>[2x]MVGLEDDTERERSPVVENGFSNGSRSSSSSAGVLSPSRKVTQGNDTLSYANILRARNKFADALALYEAMLEKDSKNVEAHIGKGICLQTQNKGNLAFDCFSEAIRLDPHNACALTHCGILHKEEGRLVEAAESYQKALMADASYKPAAECLAIVLTDLGTSLKLAGNTQEGIQKYYEALKIDPHYAPAYYNLGVVYSEMMQYDNALSCYEKAALERPMYAEAYCNMGVIYKNRGDLEMAITCYERCLAVSPNFEIAKNNMAIALTDLGTKVKLEGDVTQGVAYYKKALYYNWHYADAMYNLGVAYGEMLKFDMAIVFYELAFHFNPHCAEACNNLGVLYKDRDNLDKAVECYQMALSIKPNFAQSLNNLGVVYTVQGKMDAAASMIEKAILANPTYAEAFNNLGVLYRDAGNITMAIDAYEECLKIDPDSRNAGQNRLLAMNYINEGLDDKLFEAHRDWGWRFTRLHPQYTSWDNLKDPERPITIGYISPDFFTHSVSYFIEAPLTHHDYTKYKVVVYSAVVKADAKTYRFRDKVLKKGGVWKDIYGIDEKKIASMVREDKIDILVELTGHTANNKLGTMACRPAPVQVTWIGYPNTTGLPTVDYRITDSLADPPDTKQKQVEELVRLPDCFLCYTPSPEAGPVSPTPALSNGFVTFGSFNNLAKITPKVLQVWARILCAVPNSRLVVKCKPFCCDSIRQRFLTTLEQLGLESKRVDLLPLILFNHDHMQAYSLMDISLDTFPYAGTTTTCESLYMGVPCVTMAGSVHAHNVGVSLLTKVGLGHLVAKNEDEYVQLSVDLASDVTALSKLRMSLRDLMAGSPVCNGPSFAVGLESAYRNMWKKYCKGEVPSLRRMEMLQKEVHDDPLISKDLGPSRVSVTGEATPSLKANGSAPVPSSLPTQSPQLSKRMDSTS

Arabidopsis glycosyltransferase family 41 (GT41) protein SPINDLY (SPY) plays pleiotropic roles in plant development. Despite the amino acid sequence is similar to human O-GlcNAc transferase, Arabidopsis SPY has been identified as a novel nucleocytoplasmic protein O-fucosyltransferase. SPY-like proteins extensively exist in diverse organisms, indicating that O-fucosylation by SPY is a common way to regulate intracellular protein functions. Later studies show that SPY plays important roles in multiple developmental processes, including the circadian clock, phytohormone cytokinin signaling, plant architecture, root development, abiotic and biotic stresses.

Here, we present a crystal structure of Arabidopsis SPY/GDP complex at 2.85 Å resolution. Taken together, sequence alignment, SEC-Mals analysis and enzymatic assays collectively demonstrate that the crystal structure of engineered SPYC645S represents the conformation of wild type SPY. In the crystal structure, two SPY molecules interact with each other in a head-to-tail manner, forming a symmetrical dimer with a length of ~150 Å, a width of ~70 Å and a height of ~75 Å. Eleven tetratricopeptide repeats (TPRs) (residues 44–430) make up a superhelical conformation. The catalytic domain (residues 483–847) comprises the N-terminal lobe (N-Cat) and the C-terminal lobe (C-Cat). A short C-terminal region following the catalytic domain (residues 848–914) is invisible in the structure due to less of density map. GDP is observed on the surface of C-Cat adjacent to the interface with N-Cat. During the model building of our Arabidopsis SPY/GDP complex structure, strikingly, we found that the N-terminal loop of one protomer in a symmetry-related SPY dimer B, encompassing the residues from F20* to S37*, wrapped around the concave surface of the superhelix and traverse the active site of one protomer in the SPY dimer A. More interestingly, S21* in dimer B is located close to the phosphate groups of the GDP in one active site of dimer A, strongly suggesting it is a target residue for fucosylation. A continuous asparagine ladder throughout the inner layer of the TPR superhelix, including N300 in TPR8, N333 and N334 in TPR9, N367 and N368 in TPR10, N402 in TPR11, together with N436 in the connector region recognize the backbone of the substrate loop by forming a hydrogen-bond network. The ‘catalytic SPY’/GDP/‘substrate SPY’ complex structure and mutagenesis studies suggest a substrate-assisted catalysis, where the catalytic base is not provided by the enzyme but likely by the α-phosphate on the glycan donor substrate.> MVSVINTVDTSHEDMIHDAQMDYYGTRLATCSSDRSVKIFDVRNGGQILIADLRGHEGPVWQVAWAHPMYGNILASCSYDRKVIIWREENGTWEKSHEHAGHDSSVNSVCWAPHDYGLILACGSSDGAISLLTYTGEGQWEVKKINNAHTIGCNAVSWAPAVVPGSLIDHPSGQKPNYIKRFASGGCDNLIKLWKEEEDGQWKEEQKLEAHSDWVRDVAWAPSIGLPTSTIASCSQDGRVFIWTCDDASSNTWSPKLLHKFNDVVWHVSWSITANILAVSGGDNKVTLWKE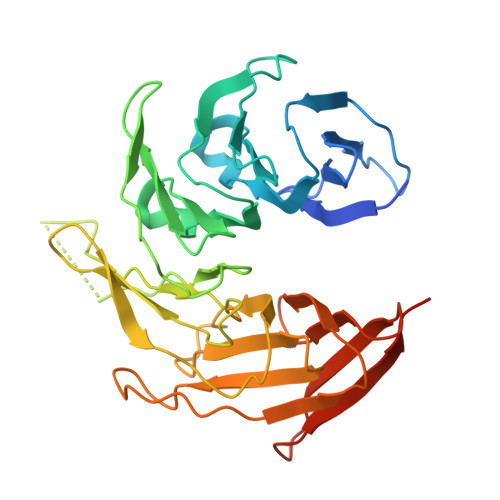SVDGQWVCISDVNKGQGSVSASVTE> KDDMKAAEQYQGAASAVDPAHVVRTNGAPDMSESEFNEA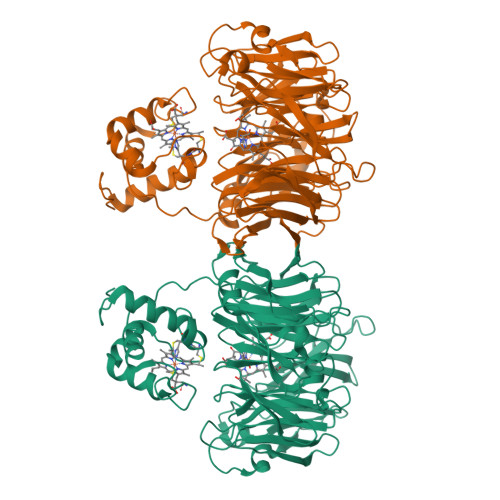KQIYFQRCAGCHGVLRKGATGKPLTPDITQQRGQQYLEALITYGTPLGMPNWGSSGELSKEQITLMAKYIQHTPPQPPEWGMPEMRESWKVLVKPEDRPKKQLNDLDLPNLFSVTLRDAGQIALVDGDSKKIVKVIDTGYAVHISRMSASGRYLLVIGRDARIDMIDLWAKEPTKVAEIKIGIEARSVESSKFKGYEDRYTIAGAYWPPQFAIMDGETLEPKQIVSTRGMTVDTQTYHPEPRVAAIIASHEHPEFIVNVKETGKVLLVNYKDIDNLTVTSIGAAPFLADGGWDSSHRYFMTAANNSNKVAVIDSKDRRLSALVDVGKTPHPGRGANFVHPKYGPVWSTSHLGDGSISLIGTDPKNHPQYAWKKVAELQGQGGGSLFIKTHPKSSHLYVDTTFNPDARISQSVAVFDLKNLDAKYQVLPIAEWADLGEGAKRVVQPEYNKRGDEVWFSVWNGKNDSSALVVVDDKTLKLKAVVKDPRLITPTGKFNVYNTQHDVY>[2x]ASYVVNNENIDKDGRQAYTGSYNRAALKQQTVKQMGPQNREAFKEDKLFKAPKNKQPIRKSENRSQNGGKQYSLNDQRTFTTIDNRTNQDEQTTATLKYDGKKAQVWVADQYITDKQAQNIGREFDERIDPLIENNFGEPSDVDNNGKVNILVYDIKDNYDQTGTYIGGYFHPRDLYNVRGSNHSEIFYMDTYPSMGTDRQHLNESQIYSTLAHEYQHMVNANENLF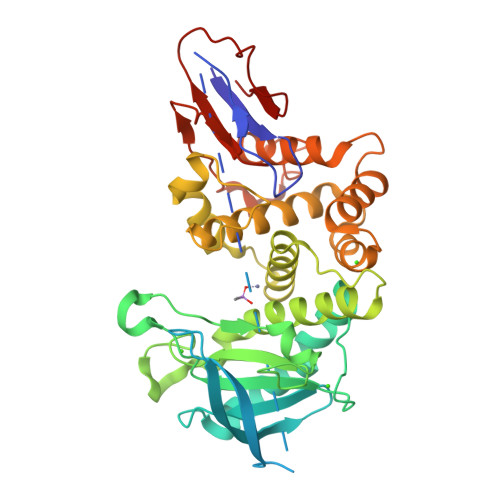KEQSQEEMDPWLNEALSMASEQMYLNAPLNSRIDYYNNSKSIAYGHSLIRWDEQGDTLSNYSLSYLFIEYLKKQSDNGEQVFKELINDPGDTNTALQNAIHEHVDPNLSLSKFMTNFRIALVKKENSGPYGFKGDADFNNVHPQPISQIPETLAPQGSVLFQTNQDFNVPNDKDEDISYNKVN> GMLSLLNTTILTPNGNEDTTADFFLTTMPTDSLSVSTLPLPEVQCFVFNVEYMNCTWQSSSEPQPTNLTLHYWYKNSDNDKVQKCSHYLFSEEITSGCQLQKKEIHLYQTFVVQLQDPREPRRQATQMLKLQNLVIPWAPENLTLHKLSESQLELNWNNRFLNHCLEHLVQYRTDWDHSWTEQSVDYRHKFSLPSVDG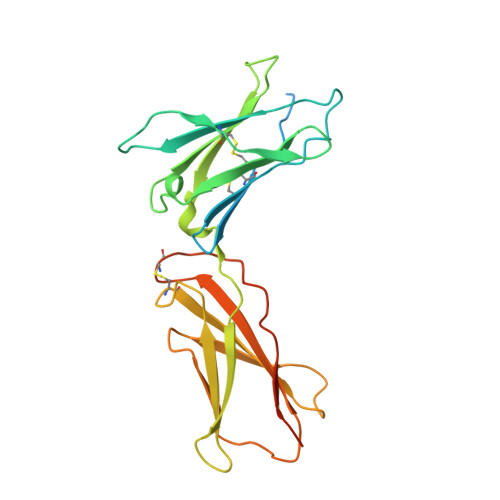QKRYTFRVRSRFNPLCGSAQHWSEWSHPIHWGSNTSKENPRTGHHHHHH> GAMGPQEYTLIKLKIHLIPEFLGSIVKGREVFVVCATLRPETMYGQTNCWILPDGEYDLVLAFDQVIPYDAKTSDGVLCKIFDKYEDTMKECNTVYICSERSAYNMAYQGIVPLIHGREQGVSDKLLPRIVSLGKVYGEQLIGTPLSAPMTPYSLIFILPMFSISMEKGTGIVTSVPSDSPDDYAALRDIKTKPLLREKYSIKDEWILDPLEIIEVPGFGFMTAELLCNQYKIQSQNDSAKLKQAKEEIYKKEFYEGILIRGKYSGMKICDAKELIRESLIKDGYALIYLE

AARSs play an essential role in protein synthesis by charging tRNAs with their cognate amino acids. Similar to other LeuRSs, the C. muris LeuRS contains a predicted editing domain exhibiting highly conserved motifs that are important for the hydrolysis of tRNALeu mischarged with noncognate amino acids, such as isoleucine or norvaline, while excluding cognate Leu-tRNALeu. The structures show the typical seven-β-strand and three-α-helix fold of the LeuRS connective polypeptide domain (CP1), plus archaeon/eukaryote-specific insertions, denoted I1ae, I2ae, I3ae, and I4ae.

Since posttransfer editing by LeuRS in apicomplexans has not been characterized, we performed binding experiments with the CmLeuRS editing domain and posttransfer editing substrate analogues for norvaline, 2-(l-norvalyl)amino-2-deoxyadenosine (Nva2AA), and isoleucine, 2-(l-isoleucyl)amino-2-deoxyadenosine (Ile2AA), which mimic a mischarged amino acid attached to Ade76. Calorimetric titrations yielded dissociation constants (Kds) of 213 and 215 μM for Nva2AA and Ile2AA, respectively, over the range of affinities observed for bacterial LeuRS, but they were lower than those seen for other editing tRNA synthetases, such as class II threonine-tRNA synthetase (ThrRS). These data, together with the conservation of important active-site residues, suggest that CmLeuRS preserves posttransfer editing activity. The posttransfer editing substrate analogues Nva2AA and Ile2AA can be unambiguously placed at the editing site of CmLeuRS. As was observed for bacterial and fungal LeuRSs, the aliphatic part of the amino acid binds into the hydrophobic pocket formed by residues T292 and V426, while the amino group interacts with the universally conserved aspartic acid (D433); the adenine base is accommodated by residues of the GTG loop (I414, S415, V423, and K418). In our structures, a water molecule is well positioned for promoting hydrolysis (3 to 4 Å to the carbon alpha atom) and is coordinated by a eukaryote-specific lysine (K496). A similarly placed water molecule is important for bacterial LeuRS editing complexes, although this is coordinated by a bacterium-specific aspartic acid (D344 in the Thermus thermophilus LeuRS). This suggests a common editing mechanism via nucleophilic attack of this water on the oxygen carbonyl, consistent with quantum mechanical calculations on LeuRS. The interactions of the catalytic water and K496 at the editing site of CmLeuRS are strikingly similar to the situation in the ThrRS-Ser3AA complex, which suggests that K496 could have a similar role in hydrolysis by eukaryotic LeuRS. Compared to the structure of the CmLeuRS-AN6426-AMP complex, the posttransfer analogues retain 3 to 4 extra water molecules (depending on the monomer chain) and a phosphate (CmLeuRS-Ile2AA complex), which mediate polar interactions between the compounds and protein residues.>[2x]FPTDDDDKIVGGYTCAANSIPYQVSLNSGSHFCGGSLINSQWVVSAAH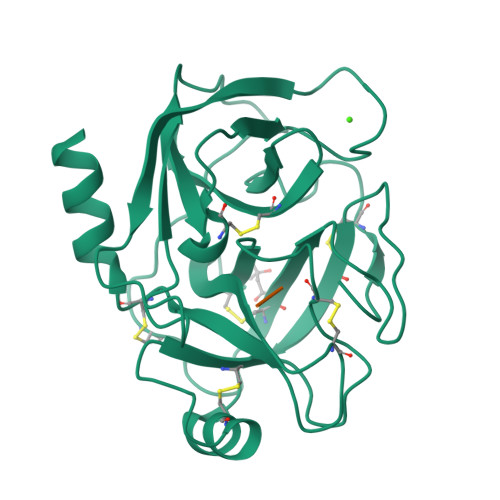CYKSRIQVRLGEHNIDVLEGNEQFINAAKIITHPNFNGNTLDNDIMLIKLSSPATLNSRVATVSLPRSCAAAGTECLISGWGNTKSSGSSYPSLLQCLKAPVLSDSSCKSSYPGQITGNMICVGFLEGGKDSCQGDSGGPVVCNGQLQGIVSWGYGCAQKNKPGVYTKVCNYVNWIQQTIAAN> MESKKRQWALEDFEIGRPLGKGKFGNVYLAREKQSKFILALKVLFKAQLEKAGVEHQLRREVEIQSHLRHPNILRLYGYFHDATRVYLILEYAPLGTVYRELQKLSKFDEQRTATYITELANALSYCHSKRVIHRDIKPENLLLGSAGELKIANFGWSVHAPSSRRTTLAGTLDYLPPEMIEGRMHDEKVDLWSLGVLCYEFLVGKPPFEANTYQETYKRISRVEFTFPDFVTEGARDLISRLLKHNPSQRPMLREVLEHPWITANSSKPSNAQNKESASKQS;> MELKEESFRDPAEVLGTGAEVDYLEQFGTSSFKESALRKQSLYLKF

Aurora‐A is a Ser/Thr protein kinase that regulates mitotic entry and mitotic spindle assembly (Nikonova et al, 2013) through phosphorylation of many substrates. These include TACC3, a member of the transforming acidic coiled‐coil family of proteins, which have conserved functions in microtubule dynamics. Like many of its other binding partners, such as TPX2, I‐2, HEF1, and N‐Myc, TACC3 is an Aurora‐A activator (Nikonova et al, 2013; Richards et al, 2016). TACC3 binds Aurora‐A through a region 30aa N‐terminal to the S558 phosphorylation site, centred on a critical phenylalanine residue, F525 (Burgess et al, 2015).

Crystals of TACC3N‐ACID bound to an Aurora‐A 122–403 C290A, C393A, D274N mutant (Aurora‐AM3KD) diffracted to 2.0 Å resolution. Residues 126–280 and 290–392 of Aurora‐AM3KD were included in the final model, with the part of the activation loop being disordered consistent with its unphosphorylated state (Cheetham et al, 2002; Burgess et al, 2016). TACC3N‐ACID mostly adopts an extended conformation but with two short regions of secondary structure: a 310‐helix formed by 528–530, and an α‐helix by 546–555 (αTR). Due to crystal packing, each molecule of TACC3N‐ACID contacts three molecules of Aurora‐AM3KD. These contacts cover the entire length of TACC3N‐ACID, which allowed it to be fully resolved, and involved three distinct sites on the surface of Aurora‐AM3KD (labelled as sites 1–3). The interaction at site 1 involves residues 523–535 of TACC3N‐ACID binding to the surface of the β‐sheet in the Aurora‐A N‐lobe contacting β‐strands β1–β3 and β5 and adopting an extended conformation, with the exception of a short 310‐helix at aa527–532. The total surface area buried in this interface is ~950 Å2, and the key contributions are made by TACC3 residues F525, L532, P528, and Aurora‐A residues I135 and R151. The F525 side chain is inserted into a pocket formed by the side chains of R151, I158, L149, E134, and main chains of G136 and A150, of Aurora‐A. The interface also involves an intermolecular salt bridge between E523 of TACC3 and R137 of Aurora‐A and a H‐bond between the main chain oxygen of TACC3 R526 and the main chain amine of Aurora‐A I135. In the complex with TACC3N‐ACID, Aurora‐AM3KD is in an inactive conformation in which the αC‐helix is distorted and K162 and E181 are separated and unable to form a salt bridge. Based upon NMR and biochemical data, we conclude that the interaction of TACC3 in solution is that observed at site 1 in the crystal structure and that this site contributes to the activation of Aurora‐A by TACC3.> MGSSHHHHHHSSGENLYFQGHMDISEWEKRYNEAYSDISKSLKKVKGIFVAYNSNIDAIKHIDEDDIEKLLEQVDAKEVQERIMEYPRQIDSPADFVARLIISMRDGKAAEVPTYTTDIHEWLTDNLGFDEARMGGQAGIISNLLANMGIKNVIAYVPWLSKEQAEYFVDSENLLHPVVENGKLELKHPKEAYNPDNKPKVNWIIEFSKGLEVKFAGEKIVVPRDNRLIVSSRPPWIRIDMSEELYEHLPEIGKNIDGAILSGYQMIKEEYEDGKTYKDYVEKAVNVIKRLKEGNPDIRIHVEFTSIQNKLIRKAILKDIVRKHVHSLGLDTVEVANALNVLGYEELAYSVIKKDENAIVALYEGAVILLHELKLERVHVHSLGYYICVVSKDSPVSPEDHRKSLLFASTVAAARALLGNINSLDDIEAGLDVPVSEQGYNQLEKLEKYLVRRGICTLED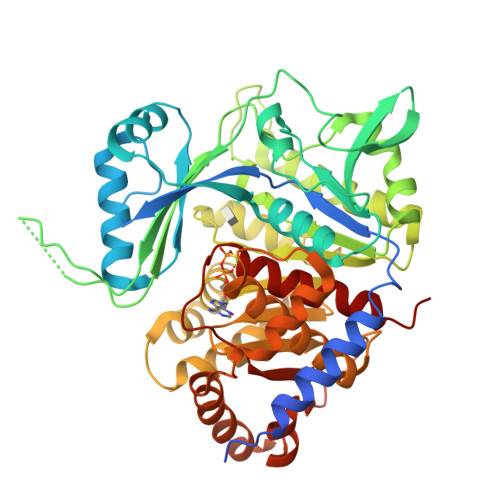FENGCICTPNHDVIIIPTKVVEKPVATVGIGDTISAAAFVSVLAKMKKKNE>MTADELVFFVNGKKVVEKNADPETTLLVYLRRKLGLCGTKLGCGEGGCGACTVMISKYDRLQNKIVHFSVNACLAPICSLHHVAVTTVEGIGNTQKLHPVQERIARSHGSQCGFCTPGIVMSMYTLLRNQPEPTVEEIENAFQGNLCRCTGYRPILQGFRTFAKDGGCCGGSGNNPNCCMNQTKDQTVSLSPSLFNPEDFKPLDPTQEPIFPPELLRLKDTPQKKLRFEGERVTWIQASTMEELLDLKAQHPDAKLVVGNTEIGIEMKFKNMLFPLIVCPAWIPELNSVVHGPEGISFGASCPLSLVESVLAEEIAKLPEQKTEVFRGVMEQLRWFAGKQVKSVASIGGNIITASPISDLNPVFMASGAKLTLVSRGTRRTVRMDHTFFPGYRKTLLRPEEILLSIEIPYSKEGEFFSAFKQASRREEDIAKVTSGMRVLFKPGTIEVQELSLCFGGMADRTISALKTTPKQLSKSWNEELLQSVCAGLAEELQLAPDAPGGMVEFRRTLTLSFFFKFYLTVLQKLGRADLEDMCGKLDPTFASATLLFQKDPPANVQLFQEVPKDQSEEDMVGRPLPHLAANMQASGEAVYCDDIPRYENELSLRLVTSTRAHAKITSIDTSEAKKVPGFVCFLTAEDVPNSNATGLFNDETVFAKDEVTCVGHIIGAVVADTPEHAQRAARGVKITYEDLPAIITIQDAINNNSFYGSEIKIEKGDLKKGFSEADNVVSGELYIGGQEHFYLETNCTIAVPKGEAGEMELFVSTQNTMKTQSFVAKMLGVPDNRIVVRVKRMGGGFGGKETRSTVVSTALALAAHKTGRPVRCMLDRDEDMLITGGRHPFLAKYKVGFMKTGTVVALEVAHFSNGGNTEDLSRSIMERALFHMDNAYKIPNIRGTGRICKTNLPSNTAFRGFGGPQGMLIAEYWMSEVAITCGLPAEEVRRKNMYKEGDLTHFNQKLEGFTLPRCWDECIASSQYLARKREVEKFN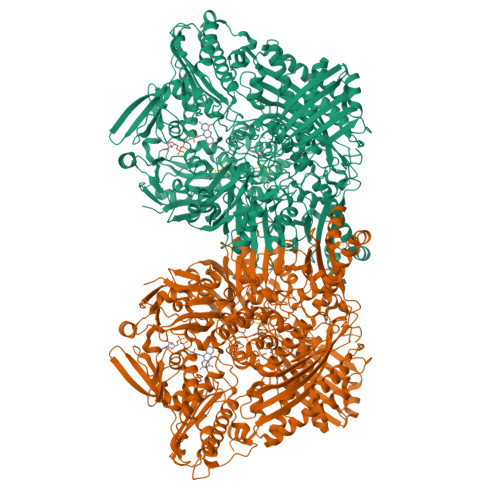RENCWKKRGLCIIPTKFGISFTLPFLNQGGALVHVYTDGSVLLTHGGTEMGQGLHTKMVQVASRALKIPTSKIHISETSTNTVPNTSPTAASASADLNGQGVYEACQTILKRLEPFKKKKPTGPWEAWVMDAYTSAVSLSATGFYKTPNLGYSFETNSGNPFHYFSYGVACSEVEIDCLTGDHKNLRTDIVMDVGSSLNPAIDIGQVEGAFVQGLGLFTMEELHYSPEGSLHTRGPSTYKIPAFGSIPIEFRVSLLRDCPNKRAIYASKAVGEPPLFLASSIFFAIKDAIRAARAQHGDNAKQLFQLDSPATPEKIRNACVDQFTTLCVTGVPENCKSWSVRI[2x]> RSMEATPIPSSETKADGILLETIS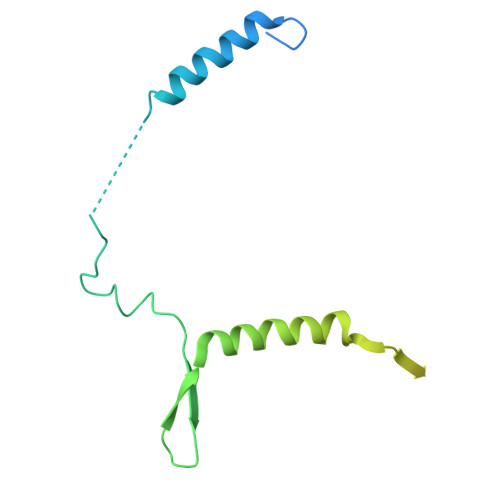VPQIRDVMERFSVLCNSNISKSRAKPVTNSSILLGKILPREEHDIAYSKDGLPNKVKTEDIRIRAQNFKSALANLEDIIFEIEKPLVVPVKLEEIKTVDPASAPNHSPEIDNLDDLVVLKKKNIQKKQPAKEKGVTEKDAVDYSKIPNILSNKPG> MSTFPGEDTRIPKRISEALSHQPLNHLVPKRELSRLLSKPVQISVQLESEDAFEEVPEELWQYPHPIDLDPLRLEESQPLRFRRPRGARLDYREDSSEIADLPGMGQLARACLSGTQLVDSAAIVESIESNAKKRKQTLAIGDVEMVSPDKKTKVMASVSPVSLNRVALGSQHLKTLERLMQ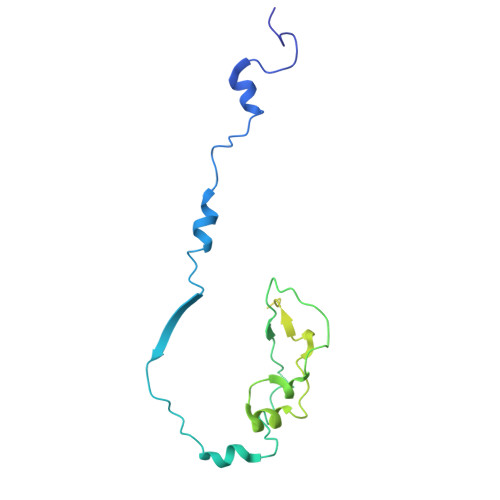YIGADESSAEFGDFEYWITLEDRATHILSEQCIDKL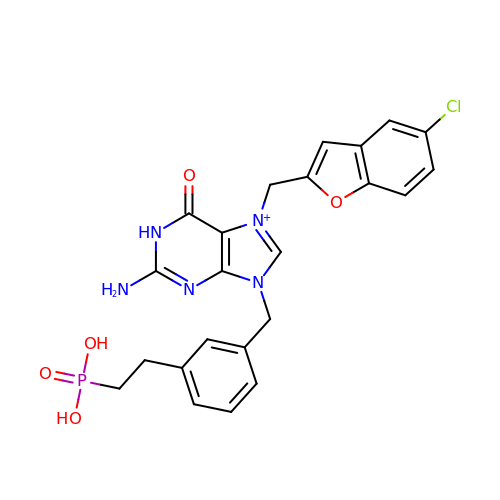2-[3-[[2-azanyl-7-[(5-chloranyl-1-benzofuran-2-yl)methyl]-6-oxidanylidene-1~{H}-purin-9-yl]methyl]phenyl]ethylphosphonic acid | C23 H22 Cl N5 O5 P | LOKWXOGCATZPBT-UHFFFAOYSA-O> ETGMPLSCSKNNSHHYIFVGNNSGLELTLTNTSLLNHKFCNLSDAHKRAQYDMALMSIVSTFHLSIPNFNQYEAMSCDFNGDNITVQYNLSHASAVDAANHCGTVANGILETFHKFFWSNNIKDAYQLPNQGKLAHCYSTSYQFLIIQNTTWEDHCTFSRPTGTKHHHHHH

The GP1 subunit of the envelope-displayed arenaviral glycoprotein spike complex (GPC) mediates host cell recognition and is an important determinant of cross-species transmission. Maturation of the GPC precursor involves proteolytic cleavage of the polyprotein into a retained and myristoylated stable signal peptide (SSP), a GP1 attachment glycoprotein, and a membrane-anchored GP2 fusion glycoprotein (1–5). We solved the crystal structures of the GP1 glycoproteins from Loei River virus (LORV), an Asiatic rodent-borne OW arenavirus of unknown pathogenicity in humans, and Whitewater Arroyo virus (WWAV), an NW arenavirus associated with spillover into human populations in North America. Both WWAV and LORV GP1s were solved at neutral pH (7.5 to 8.0) and acidic pH (5.6 to 5.0), permitting the first direct analysis of the effect of pH on the structure of GP1 in the absence of cognate GP2.

LORV GP1 crystals were generated under both neutral (pH 8.0) and acidic (pH 5.0) conditions, and X-ray diffraction data were collected to 2.5- and 2.0-Å resolution, respectively. Neutral- and acidic-pH-derived LORV GP1 structures were solved by molecular replacement, using the crystal structure of GP2-free LASV GP1 as a search model. Structural overlay analysis revealed that the two LORV GP1 structures are highly similar (0.7-Å RMSD), indicating that pH does not modulate the conformation of isolated GP1. In contrast to the structural differences observed between WWAV GP1 and other NW arenaviral GP1 glycoproteins, LORV GP1 exhibits a high level of structural conservation with other OW arenaviral GP1 glycoproteins in GP2-free states, where superimposition of LORV GP1 with LASV GP1 and Morogoro virus (MORV) GP1 resulted in a remarkably low overall RMSD (approximately 0.8 Å and 0.7 Å, respectively). In contrast to WWAV GP1, however, the structure of LORV GP1 is distinct from that likely presented on the trimeric GPC and equivalent to previously reported acidic pH structures of LASV GP1 (16) and MORV GP1 (17) in GP2-free states, which present α-DG-incompetent binding surfaces. We note that residues known to interact with α-DG in LASV GP1 are fully conserved in LORV GP1, indicative of shared receptor usage. For example, in contrast to the close spatial association of critical binding residues (H141, N146, F147, and Y150) in the GP2-associated state of LASV GP1, H139 from LORV GP1 is displaced by more than 15 Å from the nearest other predicted binding site residue (N144). Similar to previous structural analyses of LASV GP1 and MORV GP1 (16, 17), the spatial delocalization of these receptor-binding residues in LORV GP1 is consistent with the structure constituting an α-DG binding-incompetent conformation formed following detachment from GP2 during host cell entry.> MSLCRQNYHEECEAGVNKQINMEFYASYVYMSMASHFDRDDVALKGAHEFFLKSSSEEREHAMRLIKFQNQRGGRVVYQDIKKPEKDAWGTLTDAMQAALDLEKHVNQALLDLHALASKHNDPQMCDFIENHYLTEQVEAIREISGYLTNLKRCGPG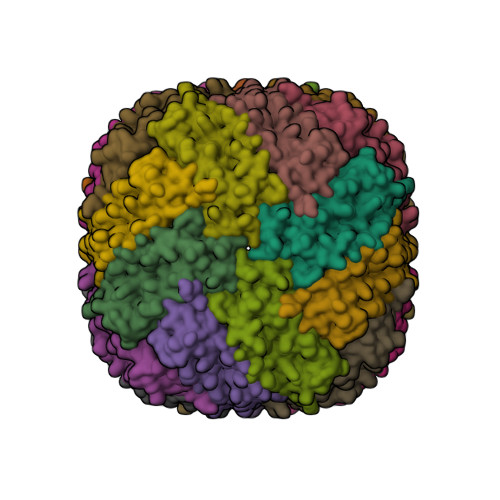LGEFLFDKELNS> NYFQGSHMFTGKALIAVKVMKPFGDWKSGDIVLVEDWKARELWEAGVVEIVDETDKIIGEIDKVIAEE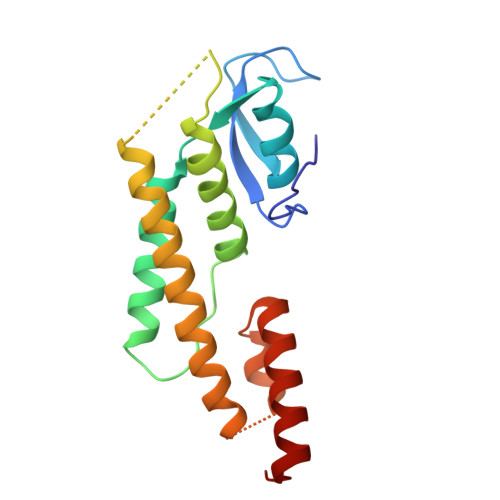RESEPLTLLPEGLYERAEFYAYYLENYVRLNPRESVDTINVKLTKLANLRKKLRDLKLIRFNKILKAVMLRPNSLELLSRLAPEERRIYLQMSKIRNEWLGDA> DYVLYKDATKPVEDRVADLLGRMTLAEKIGQMTQIERLVATPDVLRDNFIGSLLSGGGSVPRKGATAKEWQDMVDGFQKACMSTRLGIPMIYGIDAVHGQNNVYGATIFPHNVGLGATRDPYLVKRIGEATALEVRATGIQYAFAPCIAVCRDPRWGRCYESYSEDRRIVQSMTELIPGLQGDVPKDFTSGMPFVAGKNKVAACAKHFVGDGGTVDGINENNTIINREGLMNIHMPAYKNAMDKGVSTVMISYSSWNGVKMHANQDLVTGYLKDTLKFKGFVISDWEGIDRITTPAGSDYSYSVKASILAGLDMIMVPNKYQQFISILTGHVNGGVIPMSRIDDAVTRILRVKFTMGLFENPYADPAMAEQLGKQEHRDLAREAARKSLVLLKNGKTSTDAPLLPLPKKAPKILVAGSHADNLGYQCGGWTIEWQGDTGRTTVGTTILEAVKAAVDPSTVVVFAENPDAEFVKSGGFSYAIVAVGEHPYTETKGDNLNLTIPEPGLSTVQAVCGGVRCATVLISGRPVVVQPLLAASDALVAAWLPGSEGQGVTDALFGDFGFTGRLPRTWFKSVDQLPMNVGDAHYDPLFRLGYGLTTNATKKY

HvExoI releases a single Glc from non-reducing termini of oligo- and polymeric β-d-glucosides to support seed germination and plant development. HvExoI folds in an (α/β)8 barrel (domain 1) and an (α/β)6 sandwich (domain 2) that at their interface cradle a 13 Å-deep pocket- or crater-shaped active site. A vital conclusion drawn from the structural studies with the native β-d-glucan glucohydrolase, isoenzyme ExoI (HvExoI) isolated from barley seedlings, was that the glucose (Glc) product released from β-d-glucoside substrates remains entrapped in the enzyme active site until an incoming substrate binds, presumably lowering the energy barrier to facilitate Glc displacement. We discover that through chemical signalling, the incoming substrate evokes the formation of an autonomous and transient lateral cavity that serves as a conduit for the Glc product displacement from the active site.

Here, we capitalise on the Glc product entrapment observation in native HvExoI isolated from seedlings, which renders it an archetype model to examine product/substrate dissociations/associations in a pocket-shaped active site. When we first described the HvExoI structure, we were unable to explain why the trapped Glc product remained bound in the active site and has not diffused away, and what was the implication of this unassuming observation. When we first detected the Glc product entrapment in native HvExoI, we hypothesised that the role of Glc may be linked to the pre-organised state of the active site to maintain efficient catalysis required for the growth of a plant embryo.>MGSSHHHHHH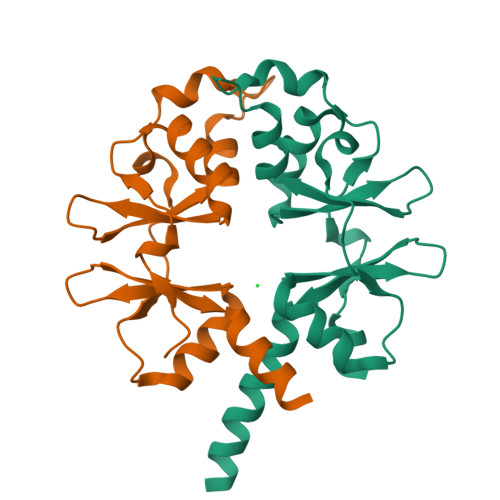SSGMISNRFGQFIDNELADSMISAEKVAHVQLGNNLEHALLVLTKCGYSVIPVLDFEFKLHGLISAAMITDAILGLERIEFERLEDLKVEDVMQTDFPVIKDFNNNERIVHLLVDHPFVCVVDSDHHFEGIVTRRVVLKQVNRYIHLQVEENR[2x]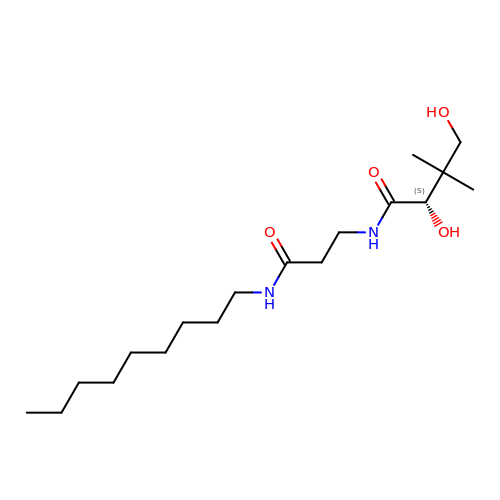(2S)-2,4-dihydroxy-3,3-dimethyl-N-[3-(nonylamino)-3-oxopropyl]butanamide | C18 H36 N2 O4 | OAZREYBYPROKTB-MRXNPFEDSA-N Bromodomain-containing protein 4 (BRD4) binds acetylated lysine residues on the N-terminal tails of histones through two bromodomains (BD1 and BD2) to regulate gene transcription. As other members of the BET family (BRD2, BRD3, and the testis-ovary specific BRDT), BRD4 has two tandem bromodomains (BD1 and BD2) and an extra C-terminal domain (ET) with a high sequence conservation through evolution. Both BRD4-BD1 and BD2 interact with acetylated lysine residues in histone and non-histone proteins to regulate a variety of cellular process including transcription, DNA replication, cell cycle progression and others. Here, we report 3′,4′,7,8-tetrahydroxyflavone (henceforth referred to as 3478), a natural product that exists in the heartwood of Acacia burkittii and Acacia acuminata, as a new inhibitor of BRD4 with a novel chemical scaffold.

Remarkably, 3478 was ∼100-fold selective for BRD4-BD2 (IC50=204 nM) than BRD4-BD1 (IC50=17.9 µM). To better understand the mechanism of different affinity activities of 3478 to BRD4-BD1 and BD2, we performed X-ray structures of 3478 in complex with BRD4-BD1 and BRD4-BD2 which were determined at resolution of 1.30 Å and 1.73 Å, respectively. 3478 binds very similarly to BRD4-BD1 and BRD4-BD2 in the binding pocket. In both structures, the carbonyl group of 3478 forms strong H-bonds with an asparagine residue (BRD4-BD1: N140, BRD4-BD2: N433), and a water molecule near the tyrosine residue (BRD4-BD1: Y97, BRD4-BD2: Y390). 7-hydroxy of 3478 forms a third H-bond with the main chain carbonyl group of a proline residue (BRD4-BD1: P82, BRD4-BD2: P375). These three H-bonds fix the 2,3‐dihydro‐1‐benzopyran‐4‐one ring tightly in the binding pocket. In contrast, its density is well defined in BD2-3478 structure, suggesting a fixed conformation and stronger interactions in BRD4-BD2. 3478 forms one additional H-bond with the water molecule near N433, and likely establishes hydrophobic interaction with His437, as NH of His437 points to two carbon atoms in its phenyl ring. The crystal structures suggest that the selectivity is mainly due to one extra hydrogen bond and the hydrophobic interaction between Histidine 437 of BD2 and phenyl group of 3478.

> SHMEQLKCCSGILKEMFAKKHAAYAWPFYKPVDVEALGLHDYCDIIKHPMDMSTIKSKLEAREYRDAQEFGADVRLMFSNCYKYNPPDHEVVAMARKLQDVFEMRFAKM> SNFKEADDAIHYRQSAFSLMAHNFGDMGAMLKGKKPFDSEIFAMRAQNVAALSKLPLEGFIPGSDQGETEALAKIWTEKSDFDAKMKTLQDNAAALLLASASDDKKLLKQSFMQVAKSCKGCHDVYKK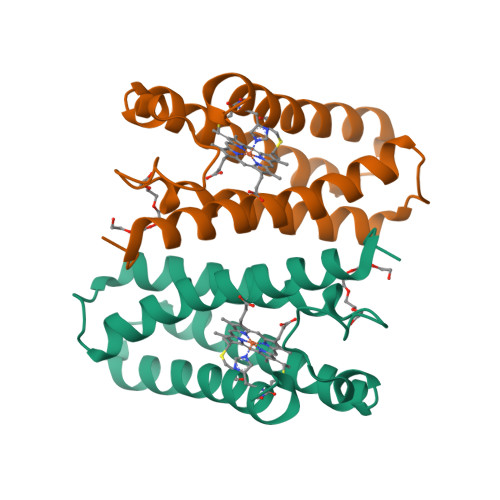D> HMPAETVRKEVALEYCRRVNAGELEGVLQLFAPDARLVD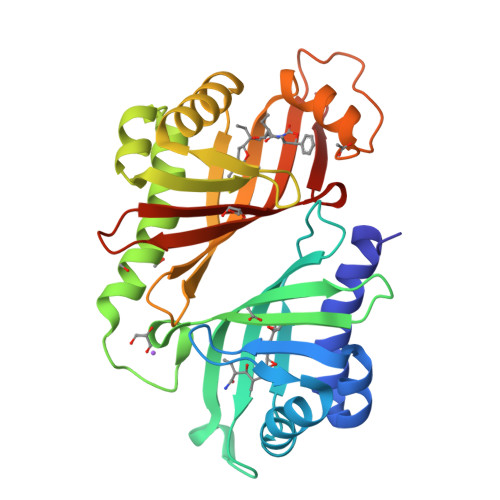PLGTEPVVGRAALAARLAPALRGAVHEEPGRPYAAHDGTSVVLPATVTVGAPGAPPQRRGRTRVMGVIEVGEDGLIREMRVMWGVTDSSWTARPAPDEERRKELAREHCLRINDGDVDGLLKLYSPRIRFEDPVGSWTRTGLEALRAHATMAVGSNVRETAGLTVAGQDGRHAAVTVSATMDYLPSGPLLARHHLMTLPAPADPHRALIGIEYVMVIGVDADGLIDEMRAYWGATDVSLLDPAA> GPLGSHMHRQPPEYNPNDEEEEEVQLKSARRATSMDLPMPMRFRHLKKTSKEAVGVY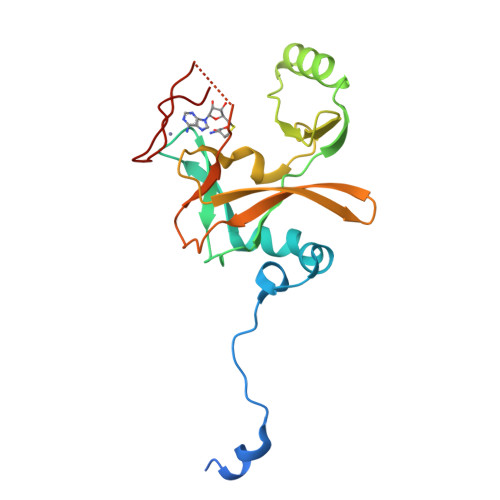RSPIHGRGLFCKRNIDAGEMVIEYAGNVIRSIQTDKREKYYDSKGIGCYMFRIDDSEVVDATMHGNAARFINHSCEPNCYSRVINIDGQKHIVIFAMRKIYRGEELTYDYKFPIEDASNKLPCNCGAKKCRKFLN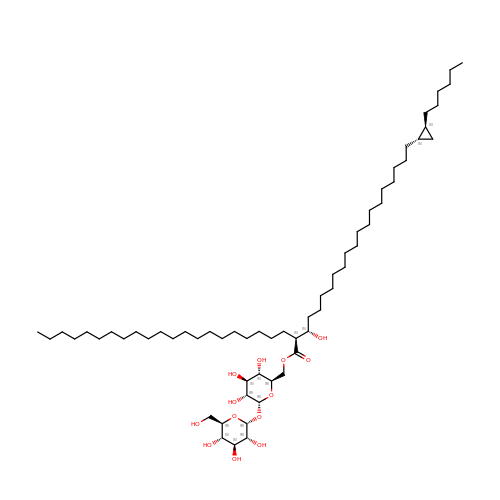6-O-[(2S)-2-{(1S)-18-[(1R,2R)-2-hexylcyclopropyl]-1-hydroxyoctadecyl}tricosanoyl]-alpha-D-glucopyranosyl alpha-D-glucopyranoside | C62 H118 O13 | UXMPVSBQNLANCZ-LXOPDUSLSA-N>[3x]MLLDEGWLAEARRVPSPHYDCRPDDENPSLLVVHNISLPPGEFGGPWIDALFTGTIDPNAHPYFAGIAHLRVSAHCLIRRDGEIVQYV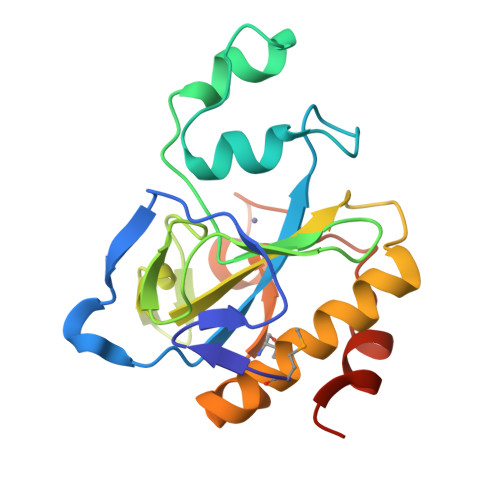PFDKRAWHAGVSSYQGRERCNDFSIGIELEGTDTLAYTDAQYQQLAAVTNALITRYPAIANNMTGHCNIAPERKTDPGPSFDWARFRALVTPSSHKEMT>[2x]ANEVIKCKAAVAWEAGKPLSIEEIEVAPPKAHEVRIKIIATAVCHTDAYTLSGADPEGCFPVILGHEGAGIVESVGEGVTKLKAGDTVIPLYIPQCGECKFCLNPKTNLCQKIRVTQGKGLMPDGTSRFTCKGKTILHYMGTSTFSEYTVVADISVAKIDPLAPLDKVCLLGCGISTGYGAAVNTAKLEPGSVCAVFGLGGVGLAVIMGCKVAG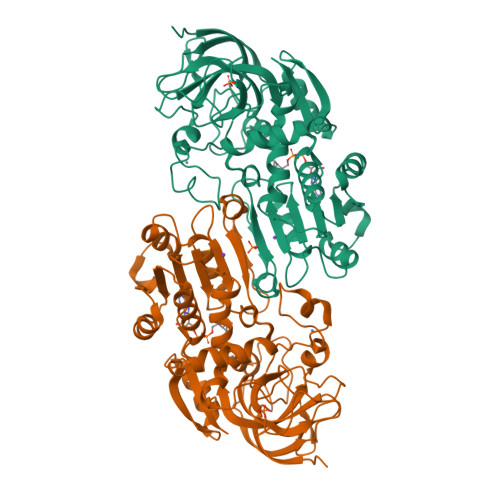ASRIIGVDINKDKFARAKEFGATECINPQDFSKPIQEVLIEMTDGGVDYSFECIGNVKVMRAALEACHKGWGVSVVVGVAASGEEIATRPFQLVTGRTWKGTAFGGWKSVESVPKLVSEYMSKKIKVDEFVTHNLSFDEINKAFELMHSGKSIRTVVKI> GQDEALNSEAAIDVCSGDDVQLANIDADSKVINVYVNKGADLSKQKLEFTLPQGATIKVNTPI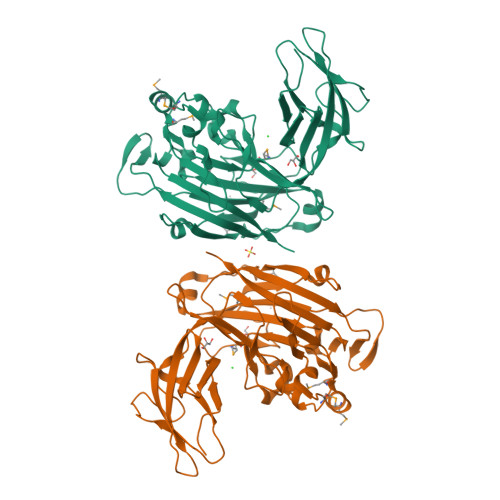TGDTESTYDFSEEPHSRKFTVTSEDGQWQPVYTVNVILAELPTLFKFEELLTTSSEYDTFYEFTPATSQEISKVLQWSSGNPGFKLTGMANSRIDYPTVQVANGFKGKAVKLETRNTGDFGAMVKMYIAAGNLFIGTFEVENALTNPRKATNFGFQFYKHPIALKGYYKFKAGEVYSVEGQPQTGKRDKCDIYAVMYEAENNSIMLNGDNVFNSDKLVLLARIEPEDIVESDEWNEFTIHFESVKGREIDDTKLQNGKYKLGIVLSSSVDGAYFRGAVGSTLYVDELELICKE> GSDASIDYNNKKSIIKKMYIFRYLTDKQCNLLIEAFRTTRYEEGDYIIQEGEVGSRFYIIKNGEVEIVKNKKRLRTLGKNDYFGERALLYDEPRTASVISKVNN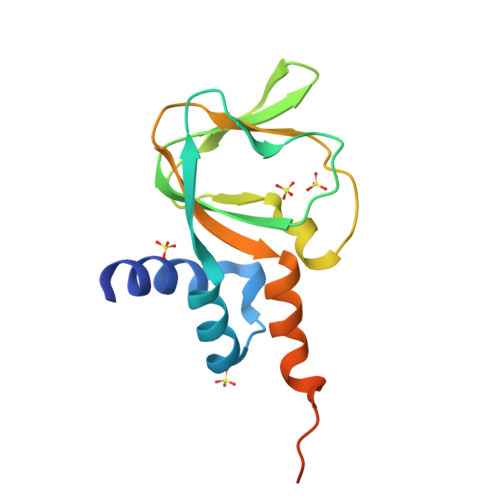VECWFVDKSVFLQIIQGPMLAHLEERIKMQDTKVEMDELE Small Hsps (sHsps) form large oligomeric assemblies with a high capacity for holding onto nonnative proteins that are handed over to the ATP-driven chaperone machines for refolding. sHsps are ubiquitous among the kingdoms of life and within mammalian genomes occur in large families with members differentially expressed in many tissues including muscle, brain and the eye lens. Small Hsp sequences have in common an “α-crystallin domain” (ACD) of around 90 amino acids, with most having a short conserved C-terminal extension bearing an I-X-I motif and a longer variable N-terminal extension. The ACD is an immunoglobulin-like beta sandwich comprising strands β2–β9, and the assembly unit is a dimer. The conserved arginine in human sHsps is on the β6 + 7 strand at the dimer interface, not far from the dyad axis.

Here we have solved the X-ray structure of the ACD dimer of human αB R120G close to physiological pH, as well as higher-resolution αB ACD wild-type controls. Therefore, the R120G mutation site was engineered into the longer L137M construct, but for simplicity, from now on the R120G/L137M structure will be referred to as R120G. There are highly ordered methyl pentane diol (MPD) molecules bound near the β6 + 7 loops and in the side pockets, where they mimic the binding of an isoleucine in the I-X-I C-terminal motif. With an interface area of 982 Å2, the R120G has a greater interface than any of the wild-type αB structures, even when the register and β6 + 7 sheet length are considered. The change in Arg120 to Gly120 results in the loss of two positive charges along the interface. This in turn results in loss of two interface ion pairs between Arg120 and Asp109 and gain of two new interface ion pairs between His83 and Asp80. Movement of these arches toward each other to form two pairs of interchain salt bridges blocks the groove. The crystal structure of R120G ACD dimer also reveals a closed groove, but in the mutant closure is caused by a pair of salt bridges between His83 and Asp80 close to the dimer 2-fold axis. The R120G with its new set of ion pairs would favour the ACD dimer in the closed form and disturb the subunit-exchange-driven assembly dynamics.

>GAMEMRLEKDRFSVNLDVKHFSPEELKVKVLGDVIEVHGKHEERQDEHGFISREFHGKYRIPADVDPLTITSSMSSDGVLTVNGPRKQVSGPER[2x]TOMUDEX | C21 H22 N4 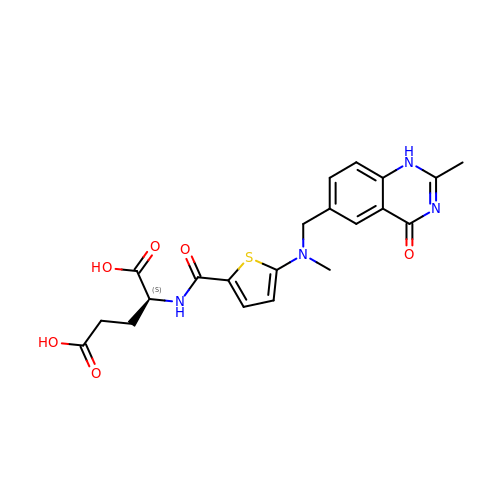O6 S | IVTVGDXNLFLDRM-HNNXBMFYSA-N> MYKLLKVKDVVRIPPRMFTMDPKEAAKIVLRETYEGIYD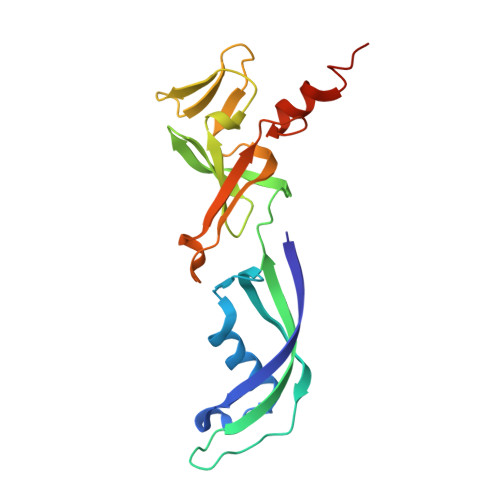RDEGVVLAILDVEEISEGVIVPGDGATYHEAIFNVLVWEPRNQEVVEGEVVEMMPYGAFIRIGPMDGLVHISQLMDDYVVFDEKNRQFIGKETNRVLKLGDYVRARIIGVSVKSRVIRENKINMTMRQPGLGKFEWIEKEKKKAKEESKGE>[2x]APAAVDWRE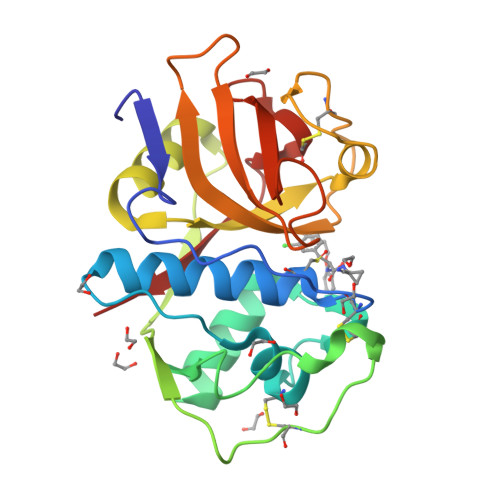KGAVTPVKDQGQCGSCWAFSTIGNIEGQWQVAGNPLVSLSEQMLVSCDTIDFGCGGGLMDNAFNWIVNSNGGNVFTEASYPYVSGNGEQPQCQMNGHEIGAAITDHVDLPQDEDAIAAYLAENGPLAIAVDATSFMDYNGGILTSCTSEQLDHGVLLVGYNDASNPPYWIIKNSWSNMWGEDGYIRIEKGTNQCLMNQAVSSAVVG Our biochemical and structural analysis of the E. coli MqsA antitoxin and the MqsR:MqsA-N complex provide a detailed 3-dimensional structural view of the free antitoxin and the TA complex. These structures combined with our biochemical data unequivocally demonstrate that MqsR, a protein previously shown to be critical for biofilm formation and the most highly upregulated gene in persister cells in E. coli, and MqsA form a novel bacterial TA system. Our data show that, as expected for a TA system, the expression of the MqsR toxin leads to growth arrest, while co-expression with its antitoxin, MqsA, rescues the growth arrest phenotype. In addition, MqsR associates with MqsA to form a tight, non-toxic complex and both MqsA alone and the MqsR:MqsA2:MqsR complex bind and regulate the mqsR promoter. MqsA itself is a two-domain protein with a novel fold that, unlike every other antitoxin, is well-ordered throughout its entire sequence and whose structure does not change upon toxin binding.

MqsA-N binds zinc and adopts a novel, elongated fold. It is composed of one long five-turn α-helix, a twisted β-sheet, loops that connect the secondary structural elements and a coordinated zinc ion. The zinc, which serves a structural and not catalytic role, is coordinated by four cysteines (Cys3, Cys6, Cys37, Cys40) with an average sulfur-zinc distance of 2.35 Å. In spite of the low sequence identity (12% identity, 18% similarity) in the MqsA-N domain among different species, these zinc-coordinated cysteines are perfectly conserved, suggesting that all bacterial MqsA proteins adopt a similar fold. The interaction between the two, long twisted β-strands and the five turn α-helix of the MqsA zinc binding domain is stabilized by an extended hydrophobic core composed of 11 residues: Ile18, Tyr20, Phe22, Leu29, Ile32, Tyr36, Met45, Phe53, Val57, Phe60 and Val64 (residues in beige). The DALI server was used to identify proteins with similar folds. Although more than 269 hits were obtained (Z-scores from 3.2 to 2.0), they aligned to only the two long β-strands and the five turn α-helix; none had the combination of strands, helix and the zinc binding pocket observed in MqsA. Thus, to the best of our knowledge, MqsA-N is a zinc binding domain with a novel fold, hereafter referred to as the MqsA fold. MqsA is also the first antitoxin described that requires a metal, zinc, for structural stability. In contrast, no shift is observed when the DNA is incubated with either MqsA-N alone or the MqsR:MqsA-N complex.

> GHMKCPVCHQGEMVSGIKDIPYTFRGRKTVLKGIHGLYCVHCEESIMNKEESDAFMAQVKAFRASVNAETVAPEFIVK> MLEEALAAIQNARDLEELKALKARYLGKKGLLTQEMKGLSALPLEERRKRGQELNAIKAALEAALEAREKALEEAALKEALERERVDVSLPGASLFSGGLHPITLMERELVEIFRALGYQAVEGPEVESEFFNFDALNIPEHHPARDMWDTFWLTGEGFRLEGPLGEEVEGRLLLRTHTSPMQVRYMVAHTPPFRIVVPGRVFRFEQTDATHEAVFHQLEGLVVGEGIAMAHLKGAIYELAQALFGPDSKVRFQPVYFPFVEPGAQFAVWWPEGGKWLELGGAGMVHPKVFQAVDAYRERLGLPPAYRGVTGFAFGLGVERLAMLRYGIPDIRYFFGGRLKFLEQFKGVL;> MRVPFSWLKAYVPELESPEVLEERLAGLGFETDRIERVFPIPRGVVFARVLEAHPIPGTRLKRLVLDAGRTVEVVSGAENARKGIGVALALPGTELPGLGQKVGERVIQGVRSFGMALSPRELGVGEYGGGLLEFPEDALPPGTPLSEAWPEEVVLDLEVTPNRPDALGLLGLARDLHALGYALVEPEAALKAEALPLPFALKVEDPEGAPHFTLGYAFGLRVAPSPLWMQRALFAAGMRPINNVVDVTNYVMLERAQPMHAFDLRFVGEGIAVRRAREGERLKTLDGVERTLHPEDLVIAGWRGEESFPLGLAGVMGGAESEVREDTEAIALEVACFDPVSIRKTARRHGLRTEASHRFERGVDPLGQVPAQRRALSLLQALAGARVAEALLEAGSPKPPEAIPFRPEYANRLLGTSYPEAEQIAILKRLGCRVEGEGPTYRVTPPSHRLDLRLEEDLVEEVARIQGYETIPLALPAFFPAPDNRGVEAPYRKEQRLREVLSGLGFQEVYTYSFMDPEDARRFRLDPPRLLLLNPLAPEKAALRTHLFPGLVRVLKENLDLDRPERALLFEVGRVFREREETHLAGLLFGEGVGLPWAKERLSGYFLLKGYLEALFARLGLAFRVEAQA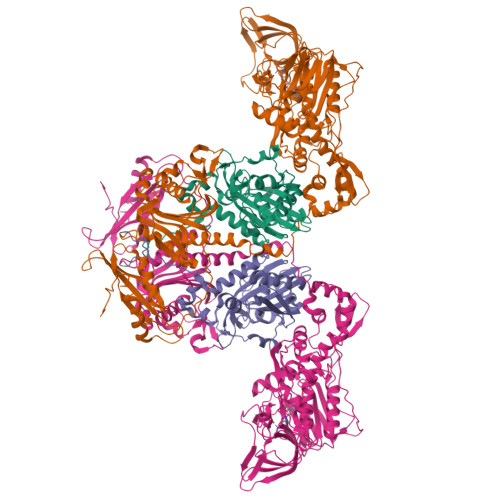FPFLHPGVSGRVLVEGEEVGFLGALHPEIAQELELPPVHLFELRLPLPDKPLAFQDPSRHPAAFRDLAVVVPAPTPYGEVEALVREAAGPYLESLALFDLYQGPPLPEGHKSLAFHLRFRHPKRTLRDEEVEEAVSRVAEALRARGFGLRGLDTP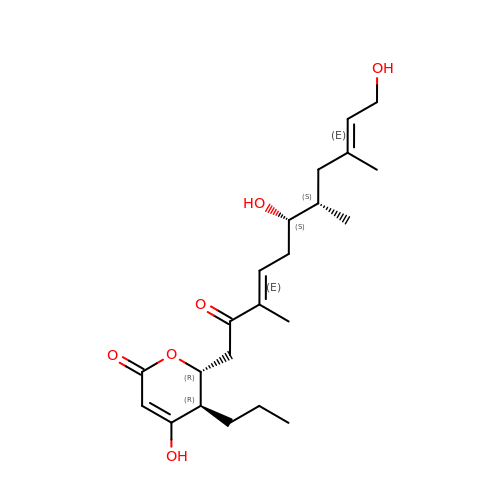(2~{R},3~{R})-4-oxidanyl-3-propyl-2-[(3~{E},6~{S},7~{S},9~{E})-3,7,9-trimethyl-6,11-bis(oxidanyl)-2-oxidanylidene-undeca-3,9-dienyl]-2,3-dihydropyran-6-one | C22 H34 O6 | UCBTXUVTSVSRBB-MHZDCPSDSA-N3,4-dihydroxy-9,10-secoandrosta-1(10),2,4-triene-9,17-dione | C19 H24 O4 | 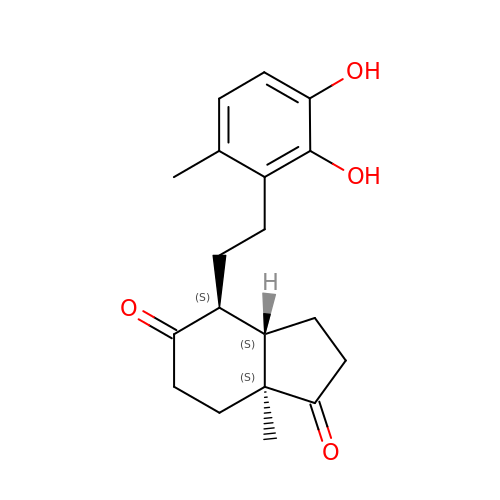YUHVBHDSVLKFNI-NJSLBKSFSA-N2-[4-(4-isoquinolin-4-ylphenyl)pyrazol-1-yl]-~{N},~{N}-dimethyl-ethanamide | C22 H20 N4 O | 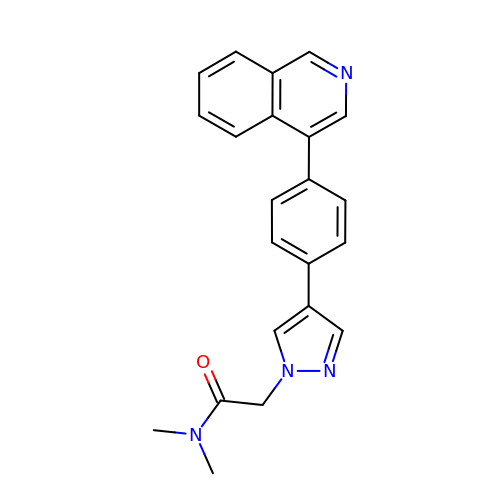WULUGQONDYDNKY-UHFFFAOYSA-N>[2x]SIEKIWAREILDSRGNPTVEVDLYTAKGL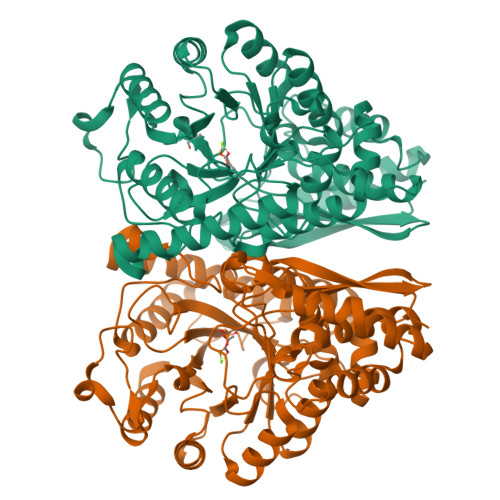FRAAVPSGASTGIYEALELRDGDKQRYLGKGVLKAVDHINSTIAPALISSGLSVVEQEKLDNLMLELDGTENKSKFGANAILGVSLAVCKAGAAERELPLYRHIAQLAGNSDLILPVPAFNVINGGSHAGNKLAMQEFMILPVGAESFRDAMRLGAEVYHTLKGVIKDKYGKDATNVGDEGGFAPNILENSEALELVKEAIDKAGYTEKIVIGMDVAASEFYRDGKYDLDFKSPTDPSRYITGDQLGALYQDFVRDYPVVSIEDPFDQDDWAAWSKFTANVGIQIVGDDLTVTNPKRIERAVEEKACNCLLLKVNQIGSVTEAIQACKLAQENGWGVMVSHRSGETEDTFIADLVVGLCTGQIKTGAPCRSERLAKYNQLMRIEEELGDEARFAGHNFRNPSVLHHHHHHHHHH(2~{R},3~{R},4~{R})-4-methyl-3-(2-oxidanylidene-2-propoxy-ethyl)sulfanyl-5-[(2~{S},3~{R})-3-oxidanyl-1-oxidanylidene-butan-2-yl]-3,4-dihydro-2~{H}-pyrrole-2-carboxylic acid | 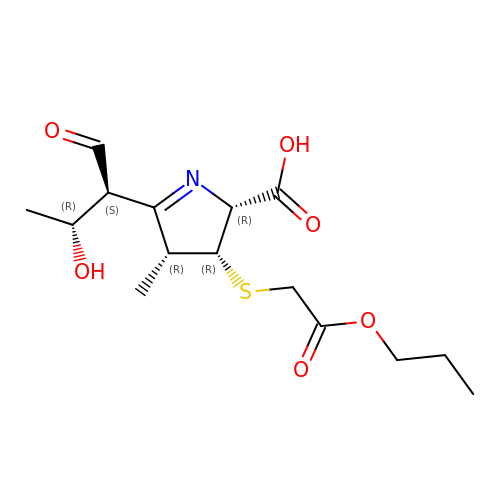C15 H23 N O6 S | ZOZKWSICEOZYLE-FDACTJFASA-N> ETPPRFTRTPVDQTGVSGGVASFICQATGDPRPKIVWNKKGKKVSNQRFEVIEFDDGSGSVLRIQPLRTPRDEAIYECVASNNVGEISVSTRLTVLREDQIPRGFPTIDMGPQLKVVERTRTATMLCAASGNPDPEITWFKDFLPVDTSNNNGRIKQLRSESIGGTPIRGALQIEQSEESDQGKYECVATNSAGTRYSAPANLYVRELREVRRVPPRFSIPPTNHEIMPGGSVNITCVAVGSPMPYVKWMLGAEDLTPEDDMPIGRNVLELNDVRQSANYTCVAMSTLGVIEAIAQITVKALPKPPGTPVVTESTATSITLTWDSGNPEPVSYYIIQHKPKNSEEPYKEIDGIATTRYSVAGLSPYSDYEFRVVAVNNIGRGPASEPVLTQKHHHHHH;> MLSGVWFLSVLTVAGILQTESRKTAKDICKIRCLCEEKENVLNINCENKGFTTVSLLQPPQYRIYQLFLNGNLLTRLYPNEFVNYSNAVTLHLGNNGLQEIRPGAFSGLKTLKRLHLNNNKLEVLREDTFLGLESLEYLQADYNYISTIEAGAFSKLNKLKVLILNDNLLLSLPSNVFRFVLLTHLDLRGNRLKVMPFAGVLEHIGGIMEIQLEENPWNCTCDLLPLKAWLDTITVFVGEIVCETPFRLHGKDVTQLTRQDLCPRKHHHHHH

Presynaptic type IIa receptor protein tyrosine phosphatases (RPTPs) (PTPδ, PTPσ and LAR in mammals) can induce synaptic differentiation by binding to various postsynaptic adhesion molecules such as IL-1 receptor accessory protein-like 1 (IL1RAPL1), IL-1 receptor accessory protein (IL-1RAcP), netrin-G ligand-3 (NGL-3), neurotrophin receptor tyrosine kinases C (TrkC) and Slit- and Trk-like (Slitrk) proteins. All Slitrk members except Slitrk3 can induce both excitatory and inhibitory synapses, whereas Slitrk3 selectively induces inhibitory synapses through binding to PTPδ7. PTPδ expressed in the developing brain consists of three immunoglobulin-like (Ig) and four fibronectin type III (Fn) domains in the extracellular region, where two splice sites exist within Ig2 and between Ig2 and Ig3. Peptide insertions (termed mini-exon peptides) at these two splice sites (referred hereafter to as meA and meB) generate splice variants of PTPδ.

After optimization of the length of PTPδ-ECD, we finally determined the crystal structure of a complex between Slitrk2 LRR1 and PTPδ Ig1-Fn1 at 3.35 Å resolution. The asymmetric unit contains one complex, where Slitrk2 LRR1 binds to PTPδ Ig1-Fn1 at a ratio of 1:1. PTPδ Ig1-2 forms a compact V-shaped unit, similarly to LAR or PTPσ Ig1-215. Ig3 is spatially separated from Ig1-2 by meB. Slitrk2 LRR1 comprises a central LRR with seven parallel β-strands flanked by N- and C-terminal caps, which are stabilized by disulfide bonds. The concave surface of Slitrk2 LRR1 surrounds two strands in PTPδ Ig2 and meB (234ELRE237) with a buried surface area of 644 Å2. Asp167 and Glu215 of Slitrk2 hydrogen bond with Arg236 of PTPδ (the third residue of meB). In addition, Asp142, Asn166 and Asp187 of Slitrk2 hydrogen bond with Arg233 of PTPδ (one-residue upstream of meB). Slitrk2 LRR1 also interacts with PTPδ Ig3 with a buried surface area of 450 Å2. Therefore, the present structure clearly indicates that binding of PTPδ to Slitrk2 depends on meB but not on meA.2-aminoethyl diphenylborinate | 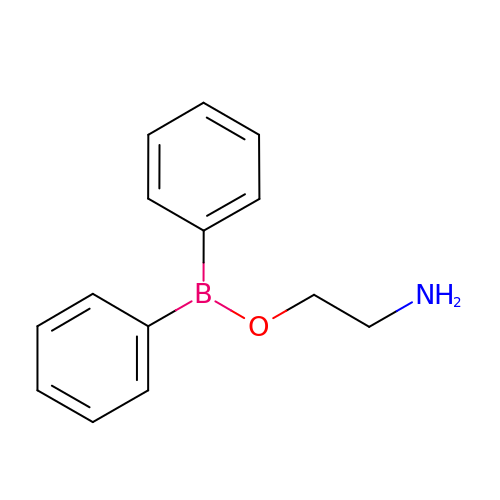C14 H16 B N O | BLZVCIGGICSWIG-UHFFFAOYSA-N>ASNFTQFVLVDNGGTGDVTVAPSNFANGVAEWISSNSRSQAYKVTCSVRQSSAQNRKYTIKVEVPKVATQTVGGVDLPVAAWRSYLNMELTIPIFATNSDCELIVKAMQGLLKDGNPIPSA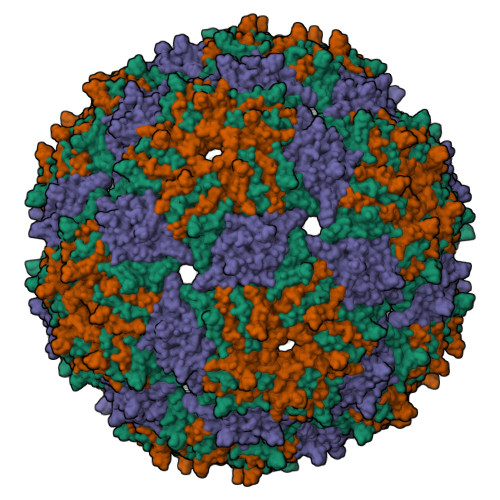IAANSGIY[3x]>QTRIAWARTELLNVCMNAKHHKEKPGPEDKLHEQCRPWRKNACCSTNTSQEAHKDVSYLYRFNWNHCGEMAPACKRHFIQDTCLYECSPNLGPWIQQVDQSWRKERVLNVPLCKEDCE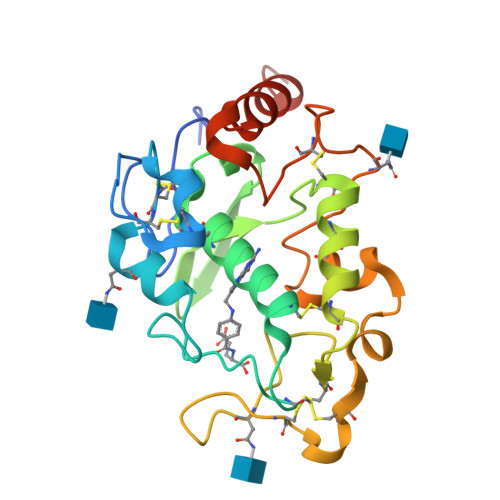QWWEDCRTSYTCKSNWHKGWNWTSGFNKCAVGAACQPFHFYFPTPTVLCNEIWTHSYKVSNYSRGSGRCIQMWFDPAQGNPNEEVARFYAAAMSGTLVPR[8x]>[2x]HMASMTGGQQMGRGSDFGDIEERGKILVSLMYSTQQGGLIVGIIRCVHLAAMDANGYSD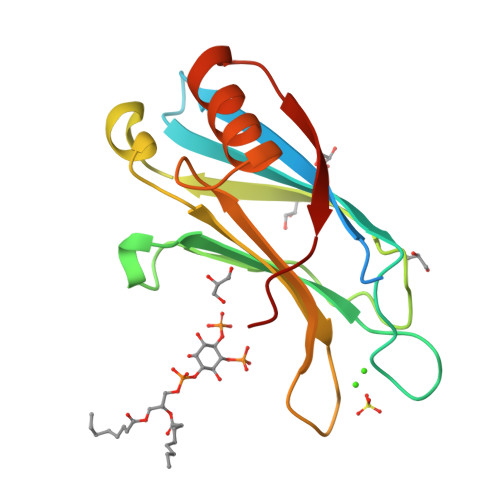PFVKLWLKPDMGKKAKHKTQIKKKTLNPEFNEEFFYDIKHSDLAKKSLDISVWDYDIGKSNDYIGGCQLGISAKGERLKHWYECLKNKDKKIERWHQLQNENH> DXLMSVEVRQ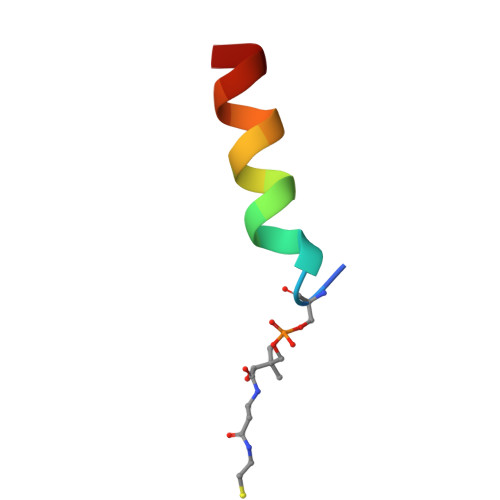TLEREL> MAGEHIKVIYFDGRGRAESIRMTLVAAGVDYEDERISFQDWPKIKPTIPGGRLPAVKVTDDHGHVKWMLESLAIARYMAKKHHMMGETDEEYYSVEKLIGQAEDVEHEYHKTLMKPQEEKEKITKEILNGKVPVLFNM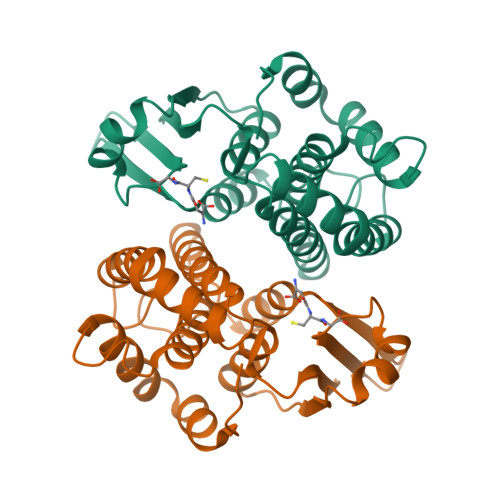ICESLKGSTGKLAVGDKVTLADLVLIAVIDHVTDLDKGFLTGKYPEIHKHRENLLASSPRLAKYLSNRPATPF> SNAMILPSFPDLTGLVVNLKFTARAEFSLNHEMAVDAFLRHSLNLGESYSHHLSIITPENGRLFYREGDTYRFVVIAMGNQQQTNSIWHTLINHLRKLPDSAPITDKQAPLRNNIKLESLNDLFDGIPVSSKESLDAYTLQRAMEQGLAWHKAANLTEQPLDIQWYWQSTVRILHADHKQHKGEQRYCRDAVQLTPLLLLKRIYETLNNVATYFGLKTNKNTTENHQAWLKEQAQYIEIQHPDLYWIDTPYFGKDAEKNTLGGMAGNFTLSLKPGIEPGLLAMLILTQMVGVGQRRTSGLGKYWLKHSLKHAHLILGLKPNRVTRSQTLLDCIIQPHIISQAIAEIEKKTNIDTLNERTLSQVQSAIGQLRKHQYQAPKLQGFTIPKKDGTERLLAVSPLYDRILQKAAAIVLTPGLDAIMSQASYGYRKGLSRQQVRYEIQNAYRQGYHWVYESDIEDFFDAVYRPQLINRLKSLLGNDPLWEQIESWLGQDIHIKDTIIERTPNLGLPQGSPLSPLLANFILDDFDSDLETHGFKIIRFADDFIILCKSQHEAQQAAHAVEQSLKEVKLSINVEKTHIIQLNQGFRFLGYLFREDHAIEIAGEKSDGRTTFAAEQTPTNLPPWLANLGTKSPQPLADDDLPKKSYGQIETQGTHLVLAGDAQIITTDNQNLIVKKDDKITHKISLEQLHAVTLIGL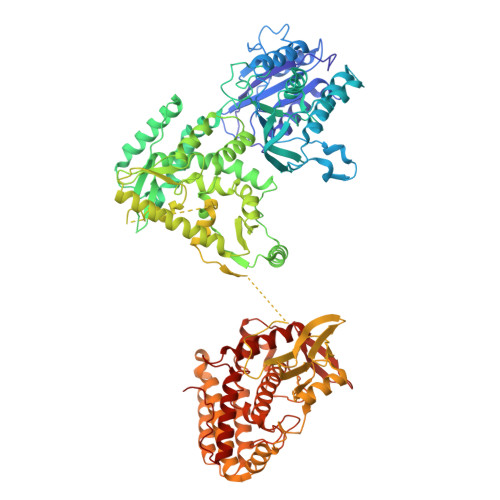HTMTLPAKHRLLEHKIPVHIADRTGRYLGAVTSFQPAQNNYKNWFIQLQMCDREPFAHAIAQQIVISRIHNQRQTLLKRKAHRKQLQQTLSNLKKLQYKVTAATKRSSLNGLEGSATREYFQQFNLFLPEWAHFSKRTRRPPKDPFNVLLSLGYTILYSHTDAILQSAGFITWKGIYHQQSAAHAALASDIMESYRHLVERYAIYIINHGQIKQDDFRQEKDHLGQDTIRLSAEARRRYVGGLINRFQKFSKDKTLHQHLYQQAQQLKNAMHNQQSSQFQVWKELK isoquinoline-1,6-diamine | C9 H9 N3 | 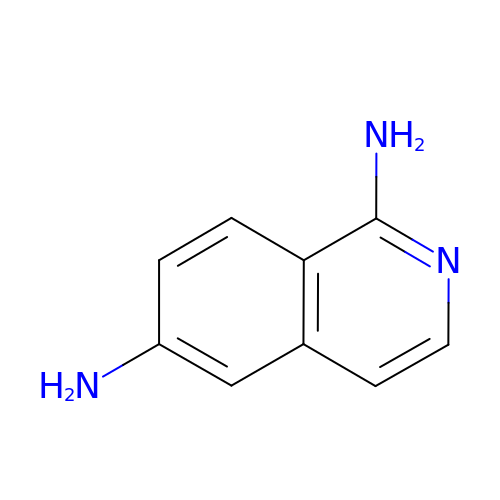FTEJISMJEPMEAC-UHFFFAOYSA-N>TPATQPLINAEPAVAAQTEQNPQVGQVMPGVQGADAPVVAQNGPSRDVKLTFAQIAPPPGSMVLRGINPNGSIEFGMRSDEVVTKAMLNLEYTPSPSLLPVQSQLKVYLNDELMGVLPVTKEQLGKKTLAQMPINPLFITDFNRVRLEFVGHYQDVCENPASTTLWLDVGRSSGLDLTYQTLNVKNDLSHFPVPFFDPRDNRTNTLPMVFAGAPDVGLQQASAIVASWFGSRSGWRGQNFPVLYNQLPDRNAIVFATNDKRPDFLRDHPAVKAPVIEMINHPQNPYVKLLVVFGRDDKDLLQAAKGIAQGNILFRGESVVVNEVKPLLPRKPYDAPNWVRTDRPVTFGELKTYEEQLQSSGLEPAAINVSLNLPPDLYLMRSTGIDMDINYRYTMPPVKDSSRMDISLNNQFLQSFNLSSKQEANRLLLRIPVLQGLLDGKTDVSIPALKLGATNQLRFDFEYMNPMPGGSVDNCITFQPVQNHVVIGDDSTIDFSKYYHFIPMPDLRAFANAGFPFSRMADLSQTITVMPKAPNEAQMETLLNTVGFIGAQTGFPAINLTVTDDGSTIQGKDADIMIIGGIPDKLKDDKQIDLLVQATESWVKTPMRQTPFPGIVPDESDRAAETRSTLTSSGAMAAVIGFQSPYNDQRSVIALLADSPRGYEMLNDAVNDSGKRATMFGSVAVIRESGINSLRVGDVYYVGHLPWFERLWYALANHPILLAVLAAISVILLAWVLWRLLRIISRRRLNPDNE[6x]

Bacterial cellulosic polymers constitute a prevalent class of biofilm matrix exopolysaccharides that are synthesized by several types of bacterial cellulose secretion (Bcs) systems, which include conserved cyclic diguanylate (c-di-GMP)-dependent cellulose synthase modules together with diverse accessory subunits. In E. coli, the biogenesis of phosphoethanolamine (pEtN)-modified cellulose relies on the BcsRQABEFG macrocomplex, encompassing inner-membrane and cytosolic subunits, and an outer membrane porin, BcsC. Here we present cryo-EM structures of the E. coli Bcs macrocomplex positioning all seven BcsRQABEFG partners and multiple c-di-GMP-binding sites.

We demonstrated previously that contrary to the canonical 1:1 BcsAB assemblies observed in purified samples from R. sphaeroides (Type III Bcs secretion system)23 and G. hansenii (Type I Bcs secretion system), in the assembled E. coli Bcs macrocomplex BcsA associates with a BcsB hexamer whose periplasmic modules of alternating carbohydrate-binding and flavodoxin-like domains (CBD1-FD1-CBD2-FD2) polymerize via a β-sheet complementation mechanism between the FD1n:FD2n+1 domains of adjacent BcsB protomers. The structure of the hexameric periplasmic crown is refined here to 2.35 Å resolution and reveals to near-atomic detail the molecular mechanism of BcsB polymerization, with more than 3300 Å2 interface surface and a free energy gain of −22.5 kcal/mol between each pair of adjacent protomers. In it, the synthase associates in a non-canonical BcsA:BcsB stoichiometry with up to six BcsB copies whose donut-shaped periplasmic modules assemble into a superhelical crown with stacking carbohydrate-binding modules likely guiding the extruded polysaccharide into the periplasm and towards the BcsC periplasmic scaffold.>MKSRIPVVLLACGSFNPITNMHLRMFEVARDHLHQTGMY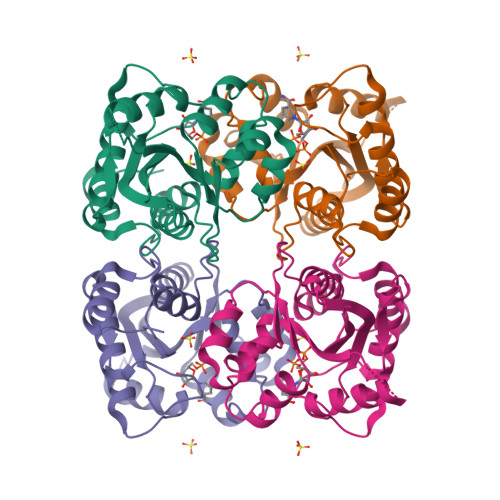QVIQGIISPVNDTYGKKDLAASHHRVAMARLALQTSDWIRVDPWESEQAQWMETVKVLRHHHSKLLRSPPQMEGPDHGKALFSTPAAVPELKLLCGADVLKTFQTPNLWKDAHIQEIVEKFGLVCVGRVSHDPKGYIAESPILRMHQHNIHLAKEPVQNEISATYIRRALGQGQSVKYLIPDAVITYIKDHGLYTKGSTWKGKSTQSTEGKTS[2x]> MGSSHHHHHHSSGLVPRGSHMSGSGSGSGTALTPSYLKDDDGRSLILRGFNTASSAKSAPDGMPQFTEADLAREYADMGTNFVRFLISWRSVEPAPGVYDQQYLDRVEDRVGWYAERGYKVMLDMHQDVYSGAITPEGNSGNGAGAIGNGAPAWATYMDGLPVEPQPRWELYYIQPGVMRAFDNFWNTTGKHPELVEHYAKAWRAVADRFADNDAVVAYDLMNEPFGGSLQGPAFEAGPLAAMYQRTTDAIRQVDQDTWVCVAPQAIGVNQGLPSGLTKIDDPRAGQQRIAYCPHLYPLPLDIGDGHEGLARTLTDVTIDAWRANTAHTARVLGDVPIILGSFGLDTTLPGARDYIERVYGTAREMGAGVSYWSSDPGPWGPYLPDGTQTLLVDTLNKPYPRAVAGTPTEWSSTSDRLQLTIEPDAAITAPTEIYLPEAGFPGDVHVEGADVVGWDRQSRLLTVRTP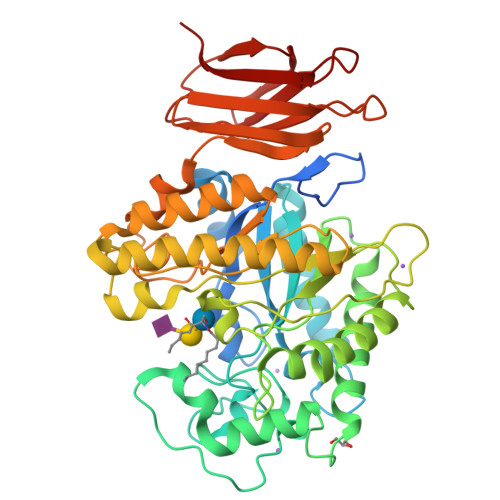ADSGNVTVTVTPAA>GLEKTVKEKLSFEGVGIHTGEYSKLIIHPEKEGTGIRFFKNGVYIPARHEFVVHTNHSTDLGFKGQRIKTVEHILSVLHLLEITNVTIEVIGNEIPILDGSGWEFYEAIRKNILNQNREIDYFVVEEPIIVEDEGRLIKAEPSDTLEVTYEGEFKNFLGRQKFTFVEGNEEEIVLARTFAFDWEIEHIKKVGLGKGGSLKNTLVLGKDKVYNPEGLRYENEPVRHKVFD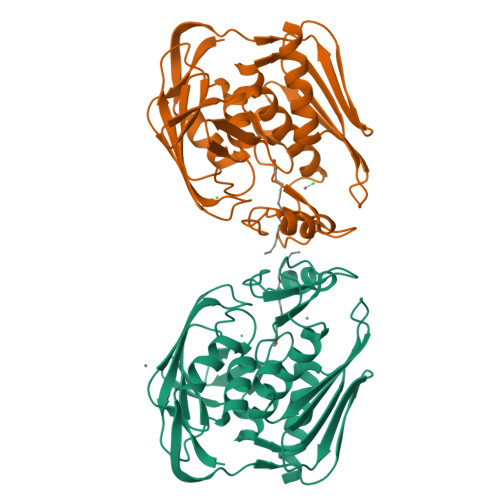LIGDLYLLGSPVKGKFYSFRGGHSLNVKLVKELAKKQKLTR[2x]> MYPGEYVPAGHNTLSSLRDELRSDLTAQSLKEAWMRVSGGMYFKSIDDYYASVDGLDQEQLGEIVSAL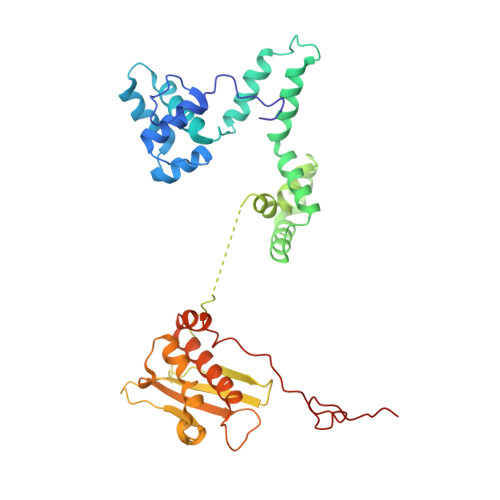LPDLRKYEAQALVTKVLESLSKPADSPSRQLSRTITADAVGLDNAPGHYTNFLEWMGRMTETKAFKTEHALFEFSRRKFNREDVRVMFENYNLMSKATLEADSTDSYSHFYTVLHDFSRKVAGEDTRHQIGVRIDPAEVDPETGIAVGHGRADGQKYMFTALIRENRDHNGSVTLLGKPLSVAFDDKSWLMEMVLMPFDEAKLDFRDFDVNLISEGKAMPSFANEIAAFACRMAVANAITKLLPLARIPLKKAGLLSVDRRREPGQFPGFVDGKKNKRKFAKR> SSIMKILLIGDVGVGKSCLLVRFVEDKFNPSFITTIGIDFKIKTVDINGKKVKLQLWDTAGQERFRTITTAYYRGAMGIILVYDVTDERTFTNIKQWFKTVNEHANDEAQLLLVGNKSDMETRVVTADQ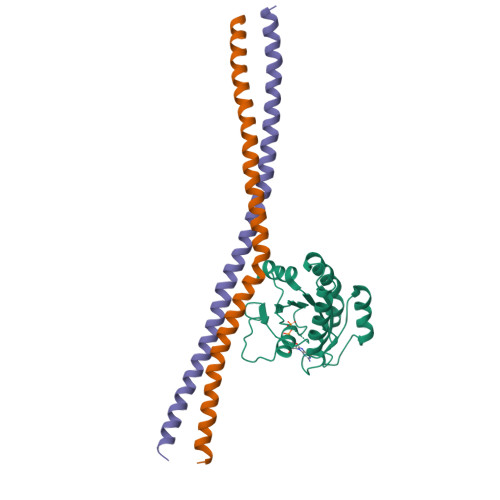GEALAKELGIPFIESSAKNDDNVNEIFFTLAKLIQEKIDSN;>[2x]SNYNQLKEDYNTLKRELSDRDDEVKRLREDIAKENELRTKAEEEADKLNKEVEDLTASLFDEANNMVADARKEKYAIEILNKRLTEQLREKDT>GSSMKASSGDQGSPPCFLRFPRPVRVVSGAEAELKCVVLGEPPPVVVWEKGGQQLAASERLSFPADGAEHGLLLTAALPTDAGVYVCRARNAAGEAYAAAAVTVLEPPA[2x];>GSSRGIPPKIEALPSDISIDEGKVLTVACAFTGEPTPEVTWSCGGRKIHSQEQGRFHIENTDDLTTLIIM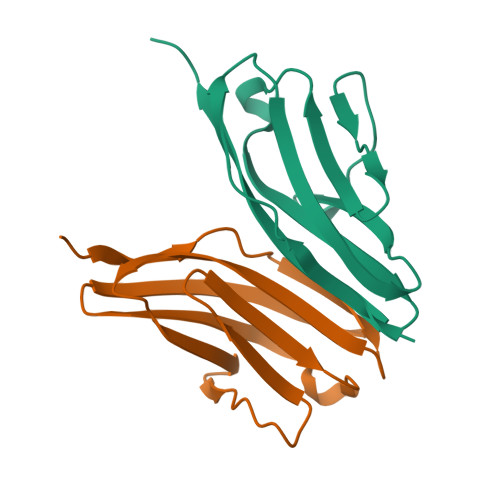DVQKQDGGLYTLSLGNEFGSDSATVNIHIRSI[2x]> MGAQVSRQNVGTHSTQ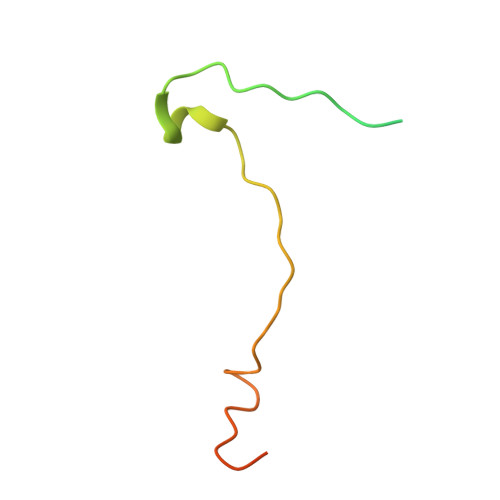NSVSNGSSLNYFNINYFKDAASNGASKLEFTQDPSKFTDPVKDVLEKGIPTLQ3,7-anhydro-2,8-dideoxy-L-glycero-D-gluco-octonic acid | C8 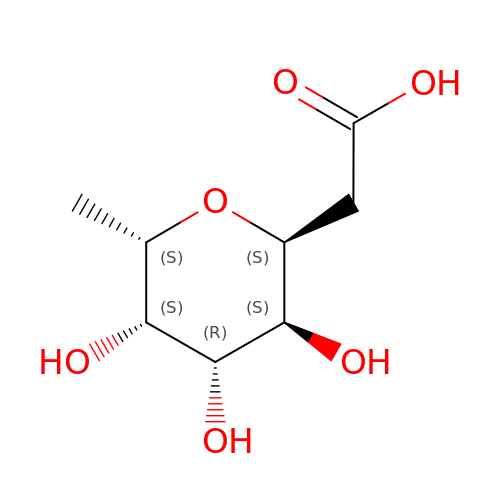H14 O6 | YTZUDUWVQZSKNN-OASCRQMUSA-N> MLAACEEPPAPAPPPAKPKAAAAVPVKAAPTETGAQAAPSYSYVYNPVGKRDPFRSPIDELGPVNANPVAACNEPLCSFDLDQLKLVA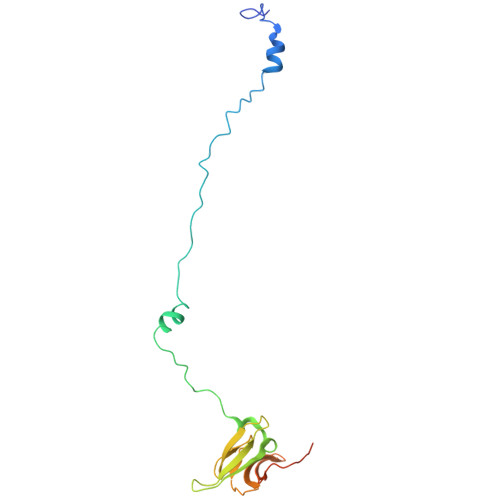VVTGDASPVAMVEDPAGRGHIVRRNTRMGRQGGKVTQILRDSVTVTEVFSGNGEIIKNPVTLQLKPDAKQDPAYNMMTGRNYGE>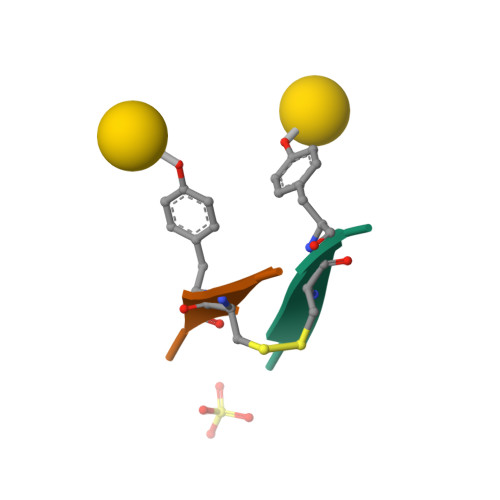[2x]YYCYY>MDDLTLRYFDAEMRYLREAGKAFAQAHPDRAAMLDLDKAGTPDPCVERLFEGFAFSMGRLRQKIDDDLPELTESLVSMLWPHYLRTIPSLSVVALTPRLSVMKMAETVPAGLEVTSRPVGPGNTVCRYRTTRAIPLNPLAVEKVVMTTEPDGRSVLKIGFACSELADWSQVDLHRLSLYLAAEAPVSSTLHLMMTKRLAALYLRLPGNDERIRIDGWFSPGGFAEEDRLWPKGDSAFSGYQLLLEYFTFREKFMFVHLNGLENVSLPAGISGFDLEVVLSQPWPADLPVTDDALCLHCVPVINLFTLEADPLIINGLESEYLLRPKRLQDGYTEIYSVDAVTGSGRTGSAEYVPFTSFRHRGGMLRHDAPERYYHTRVKRGVTGMYDTWLILGGQRWEADRMPERETLSLRITGTNGQLPRRALQSTLLDRCEQVLQAPVSVRNLCKPTLPVYPPTEDRFHWRVMSHLGTGFLNMLSSAEVLRGTLALYNWRDDELNHRRLDAILAVQHHRIQRFEKGFLLRGLDVEVTLDGNGFAGEGDIHLFGEMLNRFLALYADMNQFNQLTLIVQPEGKCIRWKENHNPRLPG[2x];> MHPVERKSQSAPARLITRYRKQLPYINFYRFCQLLEQSQPDQPPIGSGWQARQEAVRFCPYPGMGFPASEIKDAVIPEESHLP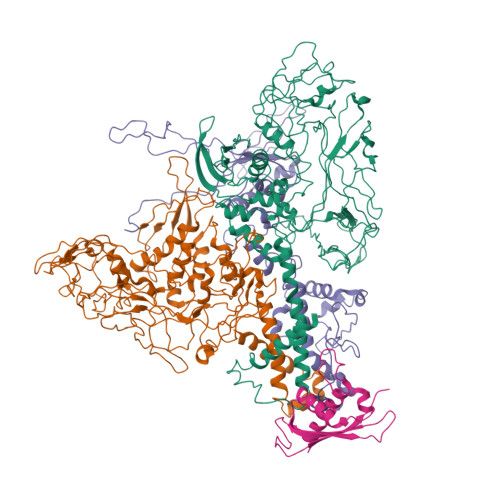PIVHVTFMGLYGVTSPLPAHYISDIAQQREGHEAAADFLDIFSHRLITQYYRIWRKYSYPATFEAGGQDKTSQYLLGLARLGIPGCAQNIATPVSRFLALLPLMLLPGRTAEGLTSLVTLLAPGTQARVWHHDRRRIPLKTPLTMRVHHPVSLKSRPVMGDHATDVNGQVLLQLSTQTGSEVQGWLPGGHLYSDLLALLHVYLGSRLDVRLQLCVERSLLPDARLSCRPAAGSPQLGRTAVMRTQAKIATSAARVMTISLGRYQRVQEHYQRKETQENGDYRW;> MPRPSLYEILYGNFTGGLELNQVGEEEQVILSVLDNMQRILNTRAGSLKHLPDYGLPDITTILQGMPGTAHQLMRVLSDVLLKYEPRIKRVDVTMQEQTQPGELHYVIDAELKDAGLVRYGTTFIPEGRVLLRHLKQQRYVQT5'-S-[2-(benzylcarbamamido)ethyl]-5'-thioadenosine 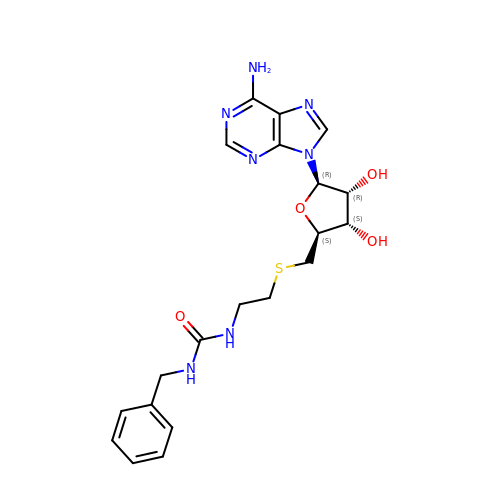| C20 H25 N7 O4 S | UTFOOFWJWOBJJY-NVQRDWNXSA-N> MALAKRIDAALIMKDGRVVKGSNFENLRDSGDPVELGKFYSEIGIDELSFWDITASVEKRKTMLELVEKVAEQIDIPFTVGGGIHDFETASELILRGADKVEINTAAVENPSLITQIAQTF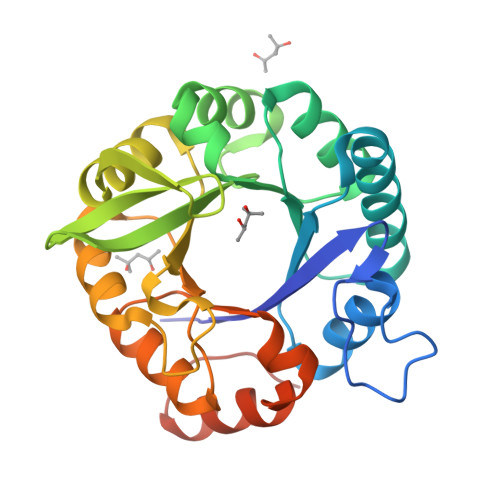GSQAVVVYIAAKRVDGEFMVFTYSGKKNTGILLRDWVVEVEKRGAGEIVLGSIDRLGTKSGYDTEMIRFVRPLTTLPIIAHRGAGKMEHFLEAFLAGADAAKADSVFHFREIDVRELKEYLKKHGVNVRLEGLGSLEHHHHHH> MASMTGGQQ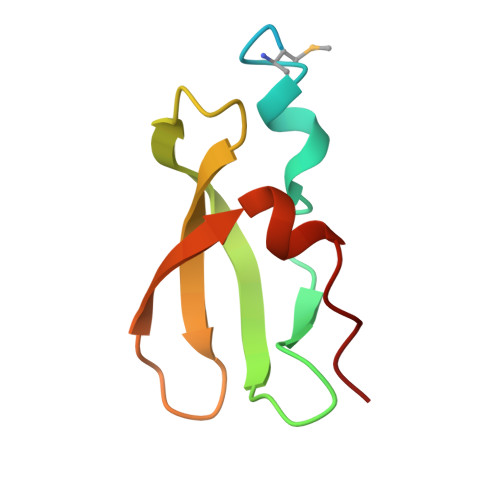MGRDPNSSSMELRQQIPTGCIKQFGQFGVPYVVGEVAEFLPDGDVLVNITLLQSGEKDIYRLSYLLEDPEAE>[4x]GKAFDDGAFTGIREINLSYNKETAIGDFQVVYDLNGSPYVGQNHSSFISGFTPVKISLDFPSEYITEVSG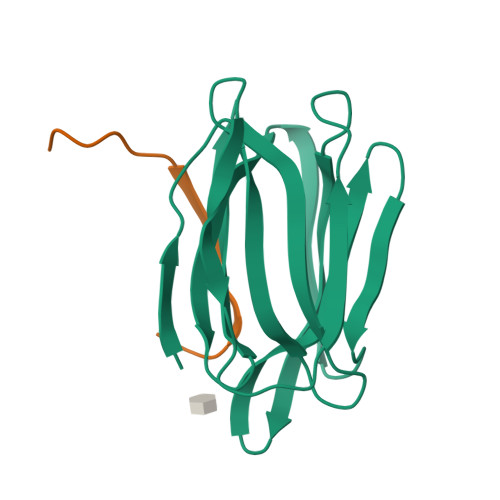YTGNVSGYVVVRSLTFKTNKKTYGPYGVTSGTPFNLPIENGLIVGFKGSIGYWMDYFSMYLSL;>[4x]DENSGKSQTVIVGPWGAKVS>MAPLKLNSRNLSQIAAAGGALVKIPTYQRGRAVKEGIVHIGVGGFHRAHLAVYIDQLMQKHGVNDYAICGVGLQPFDSAMRDALASQDHLYTLIERSAKGSFAHVIGSINSYLFAPDNREAVIAKMAHPDTKIVSLTITESGYYYNENTHELQSEHPDIQFDLDPANEKAPRTTFGFLYAGLTRRYQQGLKPFTVMSCDNMQKNGSITRHMLESFARLRNPEVAEWIAEEGAFPNAMVDRITPQTSETDKTALAEKFGIVDSWPVVTEPFTQWVIEDQFSDGRPPFEKVGVQVVKDVHAVEQFEKHKLRLLNGSHSALGYPGQLAGFQYVHEVMANPLFRKFVWQMMQEEVKPLLPEIPGVDIDEYCNTLIERFTNPTIMDQLPRICLNASGKIPQFIMPSIAEAIWETGP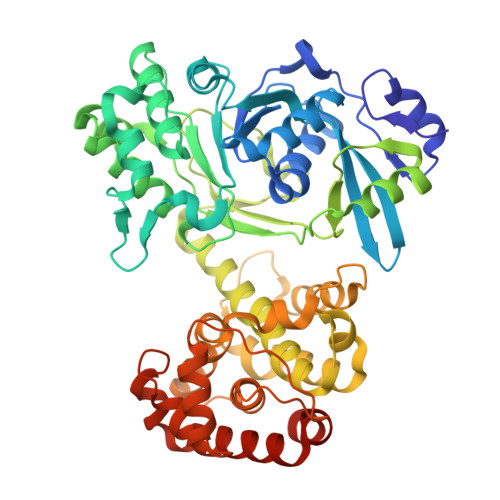FRRLCFVAAAWFHYIKGVDDRGKPFEVVDPMREELQAKARAGGNDPSELLSIKSLFGDDLRNDERFLREITTAMNDIARDGIMKTLPKYINGSHHHHHH[2x]2,3,4,5,6-pentakis(fluoranyl)phenol | C6 H F5 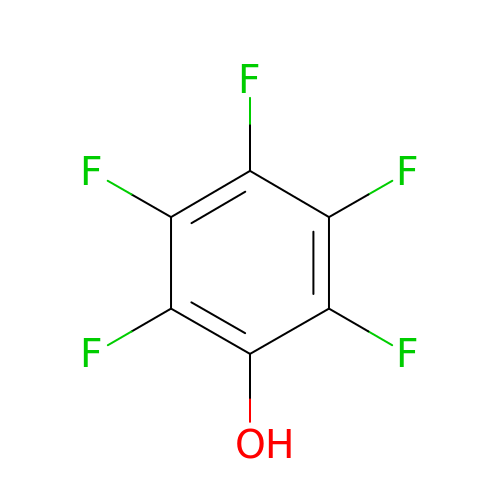O | XBNGYFFABRKICK-UHFFFAOYSA-N> VKL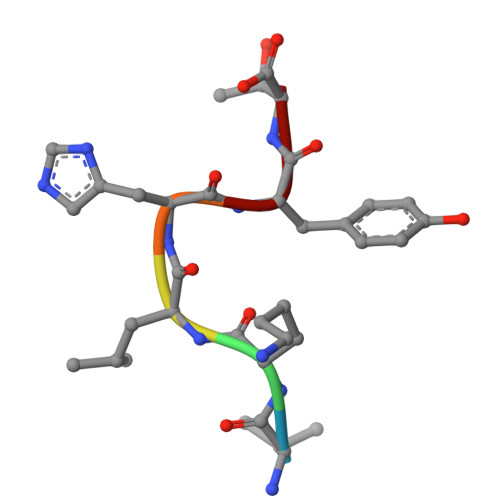HYT> IRDFNNLTKGLCTINSWHIYGKDNAVRIGEDSDVLVTREPYVSCDPDECRFYALSQGTTIRGKHSNGTIHDRSQYRALISWPLSSPPTVYNSRVECIGWSSTSCHDGKTRMSICISGPNNNASAVIWYNRRPVTEINTWARNILRTQESECVCHNGVCPVVFTDGSATGPAETRIYYFKEGKILKWEPLAGTAKHIEECSCYGERAEITCTCRDNWQGSNRPVIRIDPVAMTHTSQYICSPVLTDNPRPNDPTV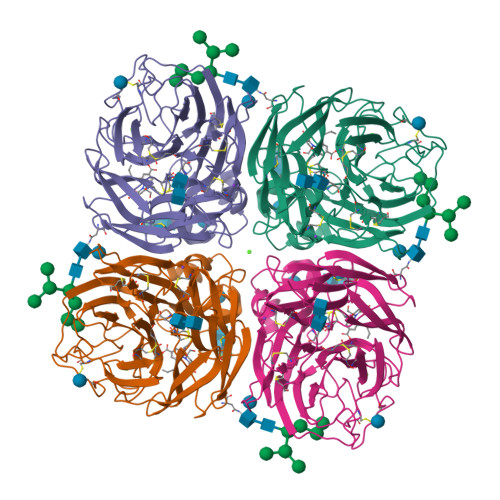GKCNDPYPGNNNNGVKGFSYLDGVNTWLGRTISIASRSGYEMLKVPNALTDDKSKPTQGQTIVLNTDWSGYSGSFMDYWAEGECYRACFYVELIRGRPKEDKVWWTSNSIVSMCSSTEFLGQWDWPDGAKIEYFL> NKYDWFEFFLNCG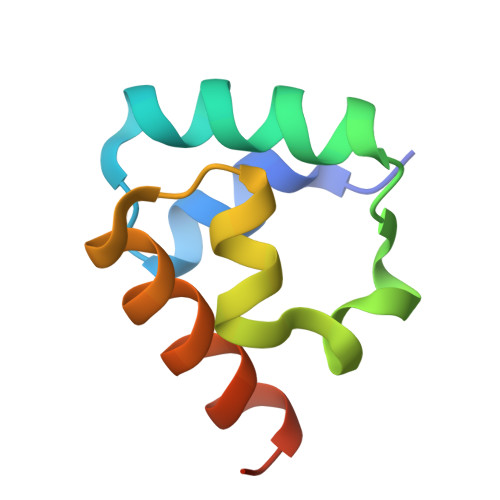VDVSNCQRYTINFDREQLTEDMMPDINNSMLRTLGLREGDIVRVMKHLDKKFGRENIAS> TCAATAGATAATAAAGGCTTACAATAGCAGCGAATAAACAGCTTGATAATAAGTA;> AGATCATTTTTTTCCATTACGCATAACGACAATGTAGAAAGGAG;> AAAACAGGAAGAAAAGCTGTCTTTATAAACAACAAGAAAATAATAAGAAC;> TGAACAATAGCAATTTGCTTTCACTCATCTGCAACGGCAT;> AGATAAGTAACTTTTTTTTTTGATCTAAAGTTTTAGTTACAAAATAAA;> GAATACGTACAAACAGCAAGAAACAATGAACCCTGAACTCACGTTGTA;> AATTGAGTAATATCAGAACAACTAAATTTGCCCTGTATGGAGATATAGCA;> TTTTTGAACACAGGGATAGCAAGCCCCCACCACCCGACGACAACCGAC;> TTATTCGGAAACAGTTAGATTAAGACGCTGTTATATAATTTAATGGGG;> TGATAGACGGTTTTTCGCCCTTTGACGTTGGAGTCCACGTTCTTTAATAGTGGACTCTTGTTCCAAACTGGAACAACACTCAACCCTATCTCGGGCTATTCTTTTGATTTATAAGGGATTTTGCCGATTTCGGAACCACCATCAAACAGGATTTTCGCCTGCTGGGGCAAACCAGCGTGGACCGCTTGCTGCAACTCTCTCAGGGCCAGGCGGTGAAGGGCAATCAGCTGTTGCCCGTCTCACTGGTGAAAAGAAAAACCACCCTGGCGCCCAATACGCAAACCGCCTCTCCCCGCGCGTTGGCCGATTCATTAATGCAGCTGGCACGACAGGTTTCCCGACTGGAAAGCGGGCAGTGAGCGCAACGCAATTAATGTGAGTTAGCTCACTCATTAGGCACCCCAGGCTTTACACTTTATGCTTCCGGCTCGTATGTTGTGTGGAATTGTGAGCGGATAACAATTTCACACAGGAAACAGCTATGACCATGATTACGAATTCGAGCTCGGTACCCGGGGATCCTCTAGAGTCGACCTGCAGGCATGCAAGCTTGGCACTGGCCGTCGTTTTACAACGTCGTGACTGGGAAAACCCTGGCGTTACCCAACTTAATCGCCTTGCAGCACATCCCCCTTTCGCCAGCTGGCGTAATAGCGAAGAGGCCCGCACCGATCGCCCTTCCCAACAGTTGCGCAGCCTGAATGGCGAATGGCGCTTTGCCTGGTTTCCGGCACCAGAAGCGGTGCCGGAAAGCTGGCTGGAGTGCGATCTTCCTGAGGCCGATACTGTCGTCGTCCCCTCAAACTGGCAGATGCACGGTTACGATGCGCCCATCTACACCAACGTGACCTATCCCATTACGGTCAATCCGCCGTTTGTTCCCACGGAGAATCCGACGGGTTGTTACTCGCTCACATTTAATGTTGATGAAAGCTGGCTACAGGAAGGCCAGACGCGAATTATTTTTGATGGCGTTCCTATTGGTTAAAAAATGAGCTGATTTAACAAAAATTTAATGCGAATTTTAACAAAATATTAACGTTTACAATTTAAATATTTGCTTATACAATCTTCCTGTTTTTGGGGCTTTTCTGATTATCAACCGGGGTACATATGATTGACATGCTAGTTTTACGATTACCGTTCATCGATTCTCTTGTTTGCTCCAGACTCTCAGGCAATGACCTGATAGCCTTTGTAGATCTCTCAAAAATAGCTACCCTCTCCGGCATTAATTTATCAGCTAGAACGGTTGAATATCATATTGATGGTGATTTGACTGTCTCCGGCCTTTCTCACCCTTTTGAATCTTTACCTACACATTACTCAGGCATTGCATTTAAAATATATGAGGGTTCTAAAAATTTTTATCCTTGCGTTGAAATAAAGGCTTCTCCCGCAAAAGTATTACAGGGTCATAATGTTTTTGGTACAACCGATTTAGCTTTATGCTCTGAGGCTTTATTGCTTAATTTTGCTAATTCTTTGCCTTGCCTGTATGATTTATTGGATGTTAATGCTACTACTATTAGTAGAATTGATGCCACCTTTTCAGCTCGCGCCCCAAATGAAAATATAGCTAAACAGGTTATTGACCATTTGCGAAATGTATCTAATGGTCAAACTAAATCTACTCGTTCGCAGAATTGGGAATCAACTGTTATATGGAATGAAACTTCCAGACACCGTACTTTAGTTGCATATTTAAAACATGTTGAGCTACAGCATTATATTCAGCAATTAAGCTCTAAGCCATCCGCAAAAATGACCTCTTATCAAAAGGAGCAATTAAAGGTACTCTCTAATCCTGACCTGTTGGAGTTTGCTTCCGGTCTGGTTCGCTTTGAAGCTCGAATTAAAACGCGATATTTGAAGTCTTTCGGGCTTCCTCTTAATCTTTTTGATGCAATCCGCTTTGCTTCTGACTATAATAGTCAGGGTAAAGACCTGATTTTTGATTTATGGTCATTCTCGTTTTCTGAACTGTTTAAAGCATTTGAGGGGGATTCAATGAATATTTATGACGATTCCGCAGTATTGGACGCTATCCAGTCTAAACATTTTACTATTACCCCCTCTGGCAAAACTTCTTTTGCAAAAGCCTCTCGCTATTTTGGTTTTTATCGTCGTCTGGTAAACGAGGGTTATGATAGTGTTGCTCTTACTATGCCTCGTAATTCCTTTTGGCGTTATGTATCTGCATTAGTTGAATGTGGTATTCCTAAATCTCAACTGATGAATCTTTCTACCTGTAATAATGTTGTTCCGTTAGTTCGTTTTATTAACGTAGATTTTTCTTCCCAACGTCCTGACTGGTATAATGAGCCAGTTCTTAAAATCGCATAAGGTAATTCACAATGATTAAAGTTGAAATTAAACCATCTCAAGCCCAATTTACTACTCGTTCTGGTGTTTCTCGTCAGGGCAAGCCTTATTCACTGAATGAGCAGCTTTGTTACGTTGATTTGGGTAATGAATATCCGGTTCTTGTCAAGATTACTCTTGATGAAGGTCAGCCAGCCTATGCGCCTGGTCTGTACACCGTTCATCTGTCCTCTTTCAAAGTTGGTCAGTTCGGTTCCCTTATGATTGACCGTCTGCGCCTCGTTCCGGCTAAGTAACATGGAGCAGGTCGCGGATTTCGACACAATTTATCAGGCGATGATACAAATCTCCGTTGTACTTTGTTTCGCGCTTGGTATAATCGCTGGGGGTCAAAGATGAGTGTTTTAGTGTATTCTTTTGCCTCTTTCGTTTTAGGTTGGTGCCTTCGTAGTGGCATTACGTATTTTACCCGTTTAATGGAAACTTCCTCATGAAAAAGTCTTTAGTCCTCAAAGCCTCTGTAGCCGTTGCTACCCTCGTTCCGATGCTGTCTTTCGCTGCTGAGGGTGACGATCCCGCAAAAGCGGCCTTTAACTCCCTGCAAGCCTCAGCGACCGAATATATCGGTTATGCGTGGGCGATGGTTGTTGTCATTGTCGGCGCAACTATCGGTATCAAGCTGTTTAAGAAATTCACCTCGAAAGCAAGCTGATAAACCGATACAATTAAAGGCTCCTTTTGGAGCCTTTTTTTTGGAGATTTTCAACGTGAAAAAATTATTATTCGCAATTCCTTTAGTTGTTCCTTTCTATTCTCACTCCGCTGAAACTGTTGAAAGTTGTTTAGCAAAATCCCATACAGAAAATTCATTTACTAACGTCTGGAAAGACGACAAAACTTTAGATCGTTACGCTAACTATGAGGGCTGTCTGTGGAATGCTACAGGCGTTGTAGTTTGTACTGGTGACGAAACTCAGTGTTACGGTACATGGGTTCCTATTGGGCTTGCTATCCCTGAAAATGAGGGTGGTGGCTCTGAGGGTGGCGGTTCTGAGGGTGGCGGTTCTGAGGGTGGCGGTACTAAACCTCCTGAGTACGGTGATACACCTATTCCGGGCTATACTTATATCAACCCTCTCGACGGCACTTATCCGCCTGGTACTGAGCAAAACCCCGCTAATCCTAATCCTTCTCTTGAGGAGTCTCAGCCTCTTAATACTTTCATGTTTCAGAATAATAGGTTCCGAAATAGGCAGGGGGCATTAACTGTTTATACGGGCACTGTTACTCAAGGCACTGACCCCGTTAAAACTTATTACCAGTACACTCCTGTATCATCAAAAGCCATGTATGACGCTTACTGGAACGGTAAATTCAGAGACTGCGCTTTCCATTCTGGCTTTAATGAGGATTTATTTGTTTGTGAATATCAAGGCCAATCGTCTGACCTGCCTCAACCTCCTGTCAATGCTGGCGGCGGCTCTGGTGGTGGTTCTGGTGGCGGCTCTGAGGGTGGTGGCTCTGAGGGTGGCGGTTCTGAGGGTGGCGGCTCTGAGGGAGGCGGTTCCGGTGGTGGCTCTGGTTCCGGTGATTTTGATTATGAAAAGATGGCAAACGCTAATAAGGGGGCTATGACCGAAAATGCCGATGAAAACGCGCTACAGTCTGACGCTAAAGGCAAACTTGATTCTGTCGCTACTGATTACGGTGCTGCTATCGATGGTTTCATTGGTGACGTTTCCGGCCTTGCTAATGGTAATGGTGCTACTGGTGATTTTGCTGGCTCTAATTCCCAAATGGCTCAAGTCGGTGACGGTGATAATTCACCTTTAATGAATAATTTCCGTCAATATTTACCTTCCCTCCCTCAATCGGTTGAATGTCGCCCTTTTGTCTTTGGCGCTGGTAAACCATATGAATTTTCTATTGATTGTGACAAAATAAACTTATTCCGTGGTGTCTTTGCGTTTCTTTTATATGTTGCCACCTTTATGTATGTATTTTCTACGTTTGCTAACATACTGCGTAATAAGGAGTCTTAATCATGCCAGTTCTTTTGGGTATTCCGTTATTATTGCGTTTCCTCGGTTTCCTTCTGGTAACTTTGTTCGGCTATCTGCTTACTTTTCTTAAAAAGGGCTTCGGTAAGATAGCTATTGCTATTTCATTGTTTCTTGCTCTTATTATTGGGCTTAACTCAATTCTTGTGGGTTATCTCTCTGATATTAGCGCTCAATTACCCTCTGACTTTGTTCAGGGTGTTCAGTTAATTCTCCCGTCTAATGCGCTTCCCTGTTTTTATGTTATTCTCTCTGTAAAGGCTGCTATTTTCATTTTTGACGTTAAACAAAAAATCGTTTCTTATTTGGATTGGGATAAATAATATGGCTGTTTATTTTGTAACTGGCAAATTAGGCTCTGGAAAGACGCTCGTTAGCGTTGGTAAGATTCAGGATAAAATTGTAGCTGGGTGCAAAATAGCAACTAATCTTGATTTAAGGCTTCAAAACCTCCCGCAAGTCGGGAGGTTCGCTAAAACGCCTCGCGTTCTTAGAATACCGGATAAGCCTTCTATATCTGATTTGCTTGCTATTGGGCGCGGTAATGATTCCTACGATGAAAATAAAAACGGCTTGCTTGTTCTCGATGAGTGCGGTACTTGGTTTAATACCCGTTCTTGGAATGATAAGGAAAGACAGCCGATTATTGATTGGTTTCTACATGCTCGTAAATTAGGATGGGATATTATTTTTCTTGTTCAGGACTTATCTATTGTTGATAAACAGGCGCGTTCTGCATTAGCTGAACATGTTGTTTATTGTCGTCGTCTGGACAGAATTACTTTACCTTTTGTCGGTACTTTATATTCTCTTATTACTGGCTCGAAAATGCCTCTGCCTAAATTACATGTTGGCGTTGTTAAATATGGCGATTCTCAATTAAGCCCTACTGTTGAGCGTTGGCTTTATACTGGTAAGAATTTGTATAACGCATATGATACTAAACAGGCTTTTTCTAGTAATTATGATTCCGGTGTTTATTCTTATTTAACGCCTTATTTATCACACGGTCGGTATTTCAAACCATTAAATTTAGGTCAGAAGATGAAATTAACTAAAATATATTTGAAAAAGTTTTCTCGCGTTCTTTGTCTTGCGATTGGATTTGCATCAGCATTTACATATAGTTATATAACCCAACCTAAGCCGGAGGTTAAAAAGGTAGTCTCTCAGACCTATGATTTTGATAAATTCACTATTGACTCTTCTCAGCGTCTTAATCTAAGCTATCGCTATGTTTTCAAGGATTCTAAGGGAAAATTAATTAATAGCGACGATTTACAGAAGCAAGGTTATTCACTCACATATATTGATTTATGTACTGTTTCCATTAAAAAAGGTAATTCAAATGAAATTGTTAAATGTAATTAATTTTGTTTTCTTGATGTTTGTTTCATCATCTTCTTTTGCTCAGGTAATTGAAATGAATAATTCGCCTCTGCGCGATTTTGTAACTTGGTATTCAAAGCAATCAGGCGAATCCGTTATTGTTTCTCCCGATGTAAAAGGTACTGTTACTGTATATTCATCTGACGTTAAACCTGAAAATCTACGCAATTTCTTTATTTCTGTTTTACGTGCAAATAATTTTGATATGGTAGGTTCTAACCCTTCCATTATTCAGAAGTATAATCCAAACAATCAGGATTATATTGATGAATTGCCATCATCTGATAATCAGGAATATGATGATAATTCCGCTCCTTCTGGTGGTTTCTTTGTTCCGCAAAATGATAATGTTACTCAAACTTTTAAAATTAATAACGTTCGGGCAAAGGATTTAATACGAGTTGTCGAATTGTTTGTAAAGTCTAATACTTCTAAATCCTCAAATGTATTATCTATTGACGGCTCTAATCTATTAGTTGTTAGTGCTCCTAAAGATATTTTAGATAACCTTCCTCAATTCCTTTCAACTGTTGATTTGCCAACTGACCAGATATTGATTGAGGGTTTGATATTTGAGGTTCAGCAAGGTGATGCTTTAGATTTTTCATTTGCTGCTGGCTCTCAGCGTGGCACTGTTGCAGGCGGTGTTAATACTGACCGCCTCACCTCTGTTTTATCTTCTGCTGGTGGTTCGTTCGGTATTTTTAATGGCGATGTTTTAGGGCTATCAGTTCGCGCATTAAAGACTAATAGCCATTCAAAAATATTGTCTGTGCCACGTATTCTTACGCTTTCAGGTCAGAAGGGTTCTATCTCTGTTGGCCAGAATGTCCCTTTTATTACTGGTCGTGTGACTGGTGAATCTGCCAATGTAAATAATCCATTTCAGACGATTGAGCGTCAAAATGTAGGTATTTCCATGAGCGTTTTTCCTGTTGCAATGGCTGGCGGTAATATTGTTCTGGATATTACCAGCAAGGCCGATAGTTTGAGTTCTTCTACTCAGGCAAGTGATGTTATTACTAATCAAAGAAGTATTGCTACAACGGTTAATTTGCGTGATGGACAGACTCTTTTACTCGGTGGCCTCACTGATTATAAAAACACTTCTCAGGATTCTGGCGTACCGTTCCTGTCTAAAATCCCTTTAATCGGCCTCCTGTTTAGCTCCCGCTCTGATTCTAACGAGGAAAGCACGTTATACGTGCTCGTCAAAGCAACCATAGTACGCGCCCTGTAGCGGCGCATTAAGCGCGGCGGGTGTGGTGGTTACGCGCAGCGTGACCGCTACACTTGCCAGCGCCCTAGCGCCCGCTCCTTTCGCTTTCTTCCCTTCCTTTCTCGCCACGTTCGCCGGCTTTCCCCGTCAAGCTCTAAATCGGGGGCTCCCTTTAGGGTTCCGATTTAGTGCTTTACGGCACCTCGACCCCAAAAAACTTGATTTGGGTGATGGTTCACGTAGTGGGCCATCGCCC;> GCCTTGTCAGAGCCGCCACCCTCAGAACCGACCAGAACCC;> AAACGATTGGAAAATCACGGTTGAGGAACCGATTGAGGGAGGTATGGT;> GAAAGCGCAGTCCGGGGTCATAATGCCCCACCACCAACATAAAGGTGGCA;> CATACATGGCTTTTTTTTTTTTTTGATGATACAGTCTGAAACATGA;> CCCCACCCTCTGGTAATAAGTTTTAATCTGAATTTCAGACTGTAGCGC;> CAGGTCAGACCGGAACTGACAGGACGGAACCACATTAAAGCACCAG;> CCAGTAACAGGAGCCACCTCCTCATTGGTCATAGCCCCCTTAAGCAAA;> TTAAAGAACTTTTGAAATCGCGAAACCGAGCCAGAAAGACAGCAATTC;> AAAATTCAGAAGGTAAAAATTATTTGCCCGTAGCATTTTCAAAGCCAGAATG;> ACAGTTTATTGCAGTATGGTTAATTTTCGCCTGAACGCCAACTACAGAGGTTATCATCAG;> ATAAAATTTTGCTCTTTCGGAACTTTAGCGTACCGTTCCAGTAAGCGT;> AACATGTTCATGTCCAGACTCATTTTAATAACGGTCACCGTCCGACATTC;> GATAAGACTCATAGACGGATATTCATGAGCCGCCGCCAGCATCGCCTC;> CATGATACCGCCACGCACCATTACCATTAGTTTCATCGTAAACAGTGT;> AGGTACCGCCACCAATGAAACCATCGAAGTTTGCCCTATT;> GCCGTCGAGAGGGTCAGGCGCATGCTCCATATCATAAGTGAGGAAGGCGGAACAGCC;> TTTTTACTCCTCAATTTTTTTTTTTTAAGCAGTAGCGACAGAATCATAGCAGCATTAGGATGT;> TTTTTCCAAGAAGGAATTTTTTTTTTACCGAGGATTAAATAAGAATTTTTTTTTTTAAACACCG;> ATGTGAATTAAATACCCAACCAGCGCTCCGGCTTAGGTTGGGAGAAGA;> TACCTCAGAGAATAGGAAATACCAAGCTTTAATTCAGCAGCGGAACAA;> GTCAAGGCCGCGTAGAAACTTATTACTTGTCACAAAATGCTGATGCAAATAA;> TTTTTTCTTTTCATAATCCCTTGATATTTTTTTTTTTTCACAAACAAATA;> TGCCTATTAGCAAAGAAACGTCACCCTCAGCGTCACCAACTAAAACGA;> ATGAGTGTACAGAGCCACTTTTTTTTTTCACCCTCAGAGCCG;> AAGTAGAGAAGGACCGTAATGTATCACCTTCCACAGACCAACCTAGTTGCGCCC;> TTCGCCATATTAGGGTAATTGAGCGCTTAAGCCCAATACCGATAA;> ATATAATACTAGAATGTGATAATTTTAACCCAAAGACAAAATTTTTTTTTTGGGACCGACTTGAGTTTTT;> CATTTTAAAGTACACAGCGATTCCCATGTATACCGAAGCCCTTTTTGA;> CGCCATCTCAACAGTTTCAAATAAGACAAAAAGACACCACGGAATAAT;> AGCGCAAAAGGAGCTTTGCACCCGACTTGCGGGAGGTTTTAATTGCAA;> TAACCTTCCCTTAGAATCCTTGCCAATCGCATATTTTAAGTACC;> TAACGAAGGCACAGCCCTCATAGTTTTTTTTTTTTAGCCCCACAAG;> GCAGCAGATTATCAAAAACAGATAGGCAGATTATACAAGACCTAAACTATATGTATCAATAG;> AGGCAAGTCGAAATGAGGTTTAGCGGATAATAGCGGGGGAAACGCA;> TTAACCGCCATTGTATCACATCTTCTATTCTTACGCGATAGCTACATA;> CAACGCCTGTAGCAGTACTCAGCCGCGACCGAAAACTTTAGGGCTTAT;> CACCCTGTATCGGTAGGCTCCATTAGACGGTGTTTAACGTCAAAAATG;> GGGATCCGAGGGTATTGACCCCACGGAGATCCCTCA;> AACTTTGAGGTGCAGGGATTTCTTAATAATTTTTAAAGTCAGATTTAT;> GCCGTTGAACCTCCCAG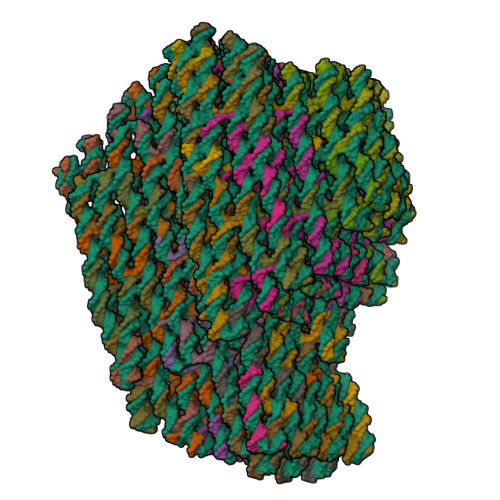CTACAATTTTATCCGATTTTTGAGAATTAAC;> GAAGCCGTACCGCATTCCAAGAATAATCGGTAAGCAGATAGCCTTTTT;> GCTTTATTTTCAAAAAAATTATCAGCAGCTATCTCCGTAACACTGAGT;> CGAACGCAATAAGTTACCTTTGGGAATTAGAGCCTTAGCGTTTGCCATTTTT;> TAGCAGCCTTTACAGTTTTTTTTTTAGAGAATAACATA;> ACTGATATAAGTATATTTTTTTTTTGCCCGGAATAGGTAGGCTGAGTTTTT;> GCGCGCGGGGACGTGCTTCGCCGCTACAGCTTTCAATAGGAATTGCGG;> TTTTTTAAATCATTCCTTTTTTTTTTGTGGGAACAAACTCAGGAAAATAGTAGTGAAAA;> GCAACATGAGGCGGTGACCGTAAGCGAGTACCACCA;> TCTTTGATTAGTAAGAGTCTGTGGGCGATCCCAGGCAACAATAACCCA;> TTTTTAACCAGAGGAATTTTTTTTTTAAACGCTCCATCACCTCATTAG;> AATGGTAGCGCCATATCGTAACAGAATCAGCACGTATAAG;> GAAAGAGAACAATGTTGGGAACCATCACGGATTAAAGTTGCAGCATTTTT;> GTTGGTCATAGCTGTTTCCTGTGTGAAAAGCCTGTTTTAACCAT;> CCATCACCAAAAACTCCGCTCACAATTCCACACTTTTTTT;> ACAAAATAATATACGAGCGTACTATGGTTTTTTTTTTTTGCTTTTGACGCTTTTT;> ACGCCAACCTGAAAGCGTAAGAAGATAGAACATATGTACCCCGGTTTG;> AGTCTACAAAAAGAACTGTTGTGAATTACCTTATAGAAATTTTT;> GGCCAACAGATACGTGGTAATGCCGGGGAAGAAGG;> CGATTAGTCTTTAATTTTTTTTTTTGCGCGAATATGATAACGGAACTGACGAGAAACACCAGTCAATA;> CTTGAGATGGTTTAAATTACCTTATTTCAAAATTAAGCTA;> AAAACGAGTAGCCGGAGAGTTCTAGCGAAAAGCCTAAAAGGGACATTCT;> CAATTTTTTTTTTATCAACGTAACAAAGCTGCTCATTCAGTA;> TTTTTACGAGACAAAATTCCTCATATATTTTATTTTATTTTA;> TATGACCCTGAAATCGGTCTGGCCTTACCTACATTTGACGAGAGCGGGAGCTATTTTT;> CATATCCAAAAGAAATTAGCAACGCAAGGAGTTAAATCTAAATT;> ATTTTATCCTCGTTCGTGCATCTGGTGTAGCACCAGCACTCAGAGCAA;> AATTATTTTTTTTTTAAATTCGCATTTCGGATTCACAGGCAATAGCATTAGG;> TTTTTTCAATCGTTGTACCAACCTAATTTTTTTTTTAACATCGCCATTAAGATTTTCGAGCGG;> ATCAAAGCGGTATATTTTATATAACACCTCTTCGCTATCGGCCTTGCCT;> TTTTTAAAATCAGGTCTTTGGCATCATTTTTTTTTTATTCTACTGATTTTTTTTTTTCGCACTCCA;> CCCGAAACATTTCGGTAGATTTGCGCAACTATTACCGCTAGCAATACT;> ATTTTTTTATTTTTAAATATGCTTTTTTTTTTAACTAAAGGGATTTTTTTTTTTGTGCTGCAAG;> TTGCTCTTCATTCCCATTTGGGCGGCACCGCGACGACAGTAAAACGCG;> TTTTTGCAACGCTAGTTTGACATATCTTTTTTTTTTTGGTCAGTTGGCACCG;> TTTTTGGTCATTGGAATTTTTTTTTTCGGTAATCGTAATATTTTGTGCAATGCTT;> CTATTTATGTCAATCCCTTCTGAAACAAGAGAATCGATCCTGAG;> TTTTTGAATGGCTACCAGTAAATTGGCAGATTCACCATTTTTTTTTTGTCACA;> GCGTTGAATGAGTGTAAAGTGTAATTGTTAAGGAAGATGATAATCATG;> TTTTTTACCGGCGCGTAAACAACCCGAAATTTTTTAAAAATTCTGAGT;> TTTAACTCGCGTCTTTTTTTTTTTGAAATGGATCACCATCAACTGTTTTTTTTTTATAGCAAACAT;> AATGTGATGGGATACTGCAGGTACGGCCAGTTTTTCTTCTTCACCGGC;> GCCAGGGCGCCGGAAGCAAGCTAACTTTTTTTTTTTCACATTAAGTGTTTTTTTTTTGACTCCAACGT;> CAAAGGGCGGGTGCCTCGCTCACTGCTTAATGTTGCATGCGGTCACGTTG;> TTTTTACGTGGCAACAGCTGAGAAGTTTTCCTTTTTTTTTTCAGTCACGACGTTGT;> GACTTCTGGTCGGTACGCAGGCCACCATTTAGAGCTTGACGGCTAAAG;> ATTGTTGTTCCGGCCAACCAGGGTGGTGCCAAGCGACAGGAAGCCGGA;> TTAGGAGGCCCAAATTAACCGTTTTTTTTTTTTGCAGCCATTTTTTT;> GAGTAGAAGGTTGGGTAACGCCTTTTTTTTTTAGGGTGTTTTTATCCA;> ATTACGAATCAGTGCAGAATCCTGATTGCCTTCACCAGGTCGAGGTATCACCCAAATCAAGTTTTTT;> AGCGAAATCGCCTGGCCCTTGCCCCAGAGTAAAATAACATCACTT;> AACCTAAGGGTTTTTTTTTTAAGAAAGCGAAAGGTCACGCTAGCTCTTTTTTTTTTGAATTCGTAAT;> CAGTGTAGCGGAGCGGGCGCTAGGGCGAAAAACCAACAAGAGTCCACT;> AACCCGCCGCGCCCGCTTTAATGAATCAGTTTGGCCTTATAAATCAAA;> TTTTTTTTTTGGGTGAGACGGGCGAGTTTTTTTTTTAAAGGGTCGTGCCGAGGATCCCCGGGTTTTT;> ACTCTAAGCTGCATTCCAGTCGCGTGAACCGTCTATCAGGGCGATGTTTTTTTTTTGCCCACTAGGA;> AAAATCAGCCCCCGGCAGGCGAAAATCCTGACGCTGGTTGAGAGAGGG;> AGGCGGTTTTTTTTTTTTTGCGTAGAGTTTTTTTTTTATAGGGTTGAGTAAAGAACTT;> TTTTTAGCGGTCCTTTTTTTTTTTTTGATGGTGGTTCAATAGCCCTTGGGC;> GGGCCGTAAAGCACTAAATTTTTTTTTTTCGGAACCGGAAAGCCGGCGATTTTT;> TCGACTGGATAGCGTCCATTTTTTTTTTATACTGCGAAATG;> GATCAAGAAAAATGATTTTTTTTTTCCATATGAATAATACATCCAATTTTT;> AAAATAGTTGCTATCCTTATCACTCATCGAATAATATCGTCAGAAGCAATATAACT;> CCCAATCCAAATAAGAAACTGAATCTAAAATCTCCATCGTAGCCGCTT;> GGTAAAGTAATTCGCTAATGCAGAACGCGCCTTTTTTTTTTTGTTTATCAACATATACTTCAATCATTTTT;> TACGAGGCCAGATACAAGGACGTTGAGAGGGTTAAAGATTCAAATATTAGCTCATTGCTGGC;> TTTAAGAGGAATATTCCTAATGAAAAGAACGAACATGGGCGCCCTGTA;> GATATAGATTTTGCAATCCTTTGATTTAGAAGTATTAGACTTTACATTAGTA;> CGAAAGCCTGCAATAGTGTTCATTTGATTTCAACTGTGTAGGAG;> GCGATTAATAGCTCAACTGGAAGTCTTTTGATCTATTATACCATCCTAGTCCTG;> GCTGGTAATATCCGAATTGAGCCAATTCTAGGTCAGGAAAAAGATGC;> ATCGGCCGGCGGATTCAGTATTGGCAAAGAGATGATGATTAACAATAA;> GTAATTAATAAAGACAGAGGCGATAAAGCTTAATACTTCG;> CCAGTTCTGAGAGCTGTTTAGCATTGCATCATTAGAGAAA;> GCCGAAAGGGTACGGTGTCATGTTTTGCGGATGGCTTAGAGCTT;> AAGGTGCGGGGTTGATTCGAAGGTTACTTTAGGAGCACTAACGTTTTA;> AATCGTCCGGATATAATAACGGACTGACCAGACGGTCAGTTACT;> CAAATATTTTTTTTTTTTTCAAACCCTCAATCATGCTGAACACCAGAAGAGGTTTAAAT;> CAACATAATAAAGCGAAGATAATTGCACGTGATGATGGCATCGGAAGT;> AACGAACTTTTTCAAATTGAGACGTCAGATGATTGCTTTGAATACCAA;> TTTTTAGGTAGAAAGATTCATCAGTACCAGACGACGATTTTTTTTTTTAAAAAC;> CAAAATAGCGAGAGGCTTTTGCGTTAATAATAGGAATAATA;> TATAAGCAAAAGGGGAAGCCTTTTTTTAATATTTCAATCATATGCGGG;> CAAAACGTTAAAACTAGCTTGAGAGATCTGGAGCTCATTGAATCCCCCTCGAATCG;> AACTTTTTTTTTTAATTCGACAACTTTTAAAACATCGC;> AACCCTCGTTTTGAGATTAACGAACTATTCAACCCAGTCAAATTATTT;> TTTATCAAAATCATAGGTCTTTTTTTTTTTGAGAGACTACCTATAAGG;> GTTTTAGTATTACCTGAGAAAATTATAACAGAGGGTGCCACGTGAGGG;> ATAAATCACAGACACCACATTCAACTAATGAT;> CGAACGTTATTAATCGTATTATAAACAACTGAATTTTGTCGTCTTTCCAGACG;> GTTTTTTTTTGTTTGAGTAACATTTACCTTTTGAGGCG;> GCTGGCAGCTTTCGCGCGAGCAACACCGCTCCTGATTTAGAACCTGA;> TAGAACAATTACATAACAAACAATCATAATAGTACCGACAAAA;> GATGAGAAAGGTAAATTGAAATCTACAAAAGAAGAGCAACACTATCAT;> TATGTGAGTGAAGTTACAAGCCAACGATTTAACATAAATTGTAA;> ACATTTTTTTTTTTCGGGAGAAACTCATTACCGTAATCTTGACAAGAACTGACCTTGTACAG;> AATTTAATCAGCTCATTAAATGTTTAATAAATATAAAGGAAT;> CACAGAGCCTAAGGAATTAGCAAATCTTCGGTCGGTTTTAATAAGAAACCCT;> GGTACCCTGAAAGAGGTCTAAACCAATTATTTTTTTTTTAATCAAGAT;> CAACTTTGAAAGAGGTTTTTTTTTTACAGATGAACGGTCATCAAGA;> ATAGACTTCAACCAGACCACCGCGCCTCCGGTATCTAACGAGCGTCT;> CTTTAAACAGTTCGCGATTTTGGCTATCA;> TTTGAGTCGAGCTTCAAAGCGAAATATCGCCTGAGGCTACTAAAGAAG;> AGTAAGTTTTGCCAGAGGGGGTAATAGTAATACCAGTCTA;> CCAAACGGGTAAAATTTTTTTTTTTACGTAATGCCACTGCCGGAAC;> GGTGAAGTTAAAGGGAATCATTGGAAGCAAGATTAGAGAATCAACAGTT;> GCGTACCTTTTGAAATATTCTAAATATAATGCTGAACTCAAACT;> AACATACAGTATAAAAATCGCGAATTGCGTAAAATACCATCTAAAGATGGAAATTCGCCA;> TAATTTTGCTTCTGTGAATAAGGCTTGCCCAACATTATTACTTTTT;> GAACGCGATAGGCTGGCGCTATTAGGAACCGAATTCGCCTGAATATACAGTAAC;> AATTTCAACAGTTTCTTTTTTTTTTAGCGGAGTGAGAAACAACAAC;> AAGGGTGTTTGGATATAGATAAATTTACGAGCATGTTTTTTTTTTTAGAAACCAATCAACGGGTAT;> CCAACGTCTAAGAACGCGAGGCAACTAATAACTCCAACGCGAACGACA>SQPIVFYDIPSNDTLKQSPWSPNTWKIRYALNIKGIKYKTEWVEYPDIEDVVKKLGGKPTGKKPDGRDHYTVPVIYDPNTKTVVEDGIKIAKYLDDAYPDTPRLFPAGTDAFQAAFDDFVWSVTLAFPLLSLLLLDVSNSLPPRSSAYFRATREQQFGKRLEEQGGEERWQQLEAGLGKFKGYLERNGAGNDLLLMGTQGGITYSDVQIASLFVWAKVVWGEGSEKWKRLMGFHGGKWAQFCAQFAEYERAD[6x]

Glutathione transferases (GSTs; EC 2.5.1.18) constitute a large superfamily of multifunctional enzymes that are involved in phase II of xenobiotic detoxification by catalyzing the conjugation of glutathione (GSH) to a variety of electrophilic compounds. Most of the GSTs are dimeric proteins, each monomer harbouring two domains : a thioredoxin N-terminal domain containing the conserved GSH binding site (G site) and a more variable C-terminal α-helical domain (H site) usually involved in the binding of the GSH acceptor compound. The fungal specific class GSTFuA is particularly concerned by this expansion. As assumed in our recent report PcGSTFuA2, PcGSTFuA3 and PcGSTFuA1 share the same structure, which contains distinctive features when compared with canonical GST structure: (i) a new mode of dimerization, (ii) an original β-hairpin (β2’β2’’) that inhibits the formation of the regular GST dimer and acts as a lid over the G-site and (iii) a supplementary helix (α4’), between helices α4 and α5, that closes the presumed H-site.

PcGSTFuA2 crystallized in the space group C2221 with three dimers in the asymmetric unit. Global NCS restraints were imposed during refinement because diffraction limit of the crystals was 3.2 Å. Structural superpositions of apo/holo PcGSTFuA1, PcGSTFuA2 and PcGSTFuA3 unambiguously showed that PcGSTFuA2 and PcGSTFuA3 are in the holo conformation in the conditions used. The observed holo conformations can be explained by the presence of crystallization agent molecules in the G sites, which mimic some of the interactions formed by bound GSH. In the structure of PcGSTFuA2, a citrate molecule mimics the binding of GSH glycyl moiety. The citrate ion stabilization involves the main chains of Tyr-71 and Val-73 and the side-chains of Tyr-46, His-70 and Arg-154. The distance plot, which compares superposed structures of holo PcGSTFuA1 and PcGSTFuA2, reveals no big differences. The largest is localized in the center of the helix α4 where a residue is inserted in PcGSTFuA2 sequence. This difference results in a disruption in the continuity of helix α4.>[2x]GSHMAHAMENSWTISKEYHIDEEVGFALPNPQENLPDFYNDWMFIAKHLPDLIESGQLRERVEKLNMLSIDHLTDHKSQRLARLVLGCITMAYVWGKGHGDVRKVLPRNIAVPYCQLSKKLELPPILVYAD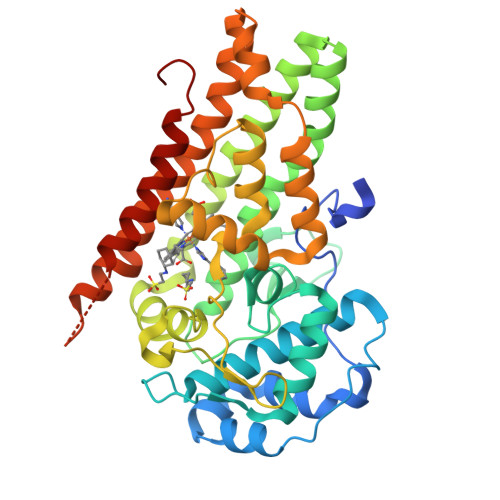CVLANWKKKDPNKPLTYENMDVLFSFRDGDCSKGFFLVSLLVEIAAASAIKVIPTVFKAMQMQERDTLLKALLEIASCLEKALQVFHQIHDHVNPKAFFSVLRIYLSGWKGNPQLSDGLVYEGFWEDPKEFAGASAGQSSVFQCFDVLLGIQQTAGGGHAAQFLQDMRRYMPPAHRNFLCSLESNPSVREFVLSKGDAGLREAYDACVKALVSLRSYHLQIVTKYILIPASQQPKENKTSEDPSKLEAKGTGGTDLMNFLKTVRSTTEKSLLKEG To overcome the issues of current PL and photo-crosslinking techniques, we here introduce a new method that can perform a photo-crosslinking reaction with proximal proteins using a visible light-activable chemical ligand (Spotlight) in a live cell. For this reason, we utilized the HaloTag system to efficiently deliver AzNP to the POI. HaloTag is an engineered tag protein that can covalently capture the haloalkane ligand within a few minutes in live cells with high efficiency. Since protein-ligand binding interactions and various “in-cell chemical reactions,” including the strain-promoted click reaction and photo–activation reactions, have been successfully realized with HaloTag, we expected HaloTag to be a suitable platform for our proximity photo-crosslinking system using an AzNP-conjugated ligand.

Among the photo-crosslinkable handles, naphthyl azide-based 4-azido-N-ethyl-1,8-naphthalimide (AzNP) attracted our interest for the following reasons: (1) it is highly stable in aqueous solutions, and has been widely used in hydrogen sulfide sensors;17,18 (2) it emits strong green fluorescence, which has been used in the fluorogenic imaging of alkyne-modified biomolecules in live mammalian cells; and (3) it shows good photo-crosslinking ability: upon UV illumination, AzNP can convert to the aryl nitrene species, which can covalently attach to proteins. To test this model, we synthesized AzNP-conjugated HaloTag ligands (VL1 and VL2) with two linker sizes (see ESI†). VL1 showed fairly strong absorbance in the visible light range (λmax = 375 nm, extinction coefficient value = 2230 M−1 cm−1; Fig. S3†). In this model system, VL1 successfully generated the photo-crosslinked product of FKBP25-HaloTag and EGFP-FRB that appeared around 120 kDa only in the presence of rapamycin and in the blue LED light illumination condition. In this reaction on the FKBP25-HaloTag, VL1 containing the PEG1 linker showed stronger crosslinking efficiency with EGFP-FRB compared with that of VL2 containing the PEG2 linker. Notably, we used an ambient blue LED household lamp (∼0.057 W cm−2) for all of our photo-crosslinking experiments in test tubes and live cells with VL1, which highlights the sensitivity of AzNP and the requirement of only low-intensity visible light illumination. We tested the specificity of AzNP-containing HaloTag ligands (VL1) to the HaloTag protein and whether it captures the local PPI network in various subcellular compartments in live cells. Since VL1 emits green fluorescence (λmax = 540 nm, Fig. S3†) and its fluorescence is increased after the photo-crosslinking reaction (Fig. S4†), we expected that targeting of VL1 and formation of POI-HaloTag could be readily tracked in real time in live cells, whereas other UV-crosslinking ligands (e.g., phenyl azide, diazirine) would not be visualized with microscope imaging due to their negligible fluorescence emission.

> SGSAEIGTGFPFDPHYVEVLGERMHYVDVGPRDGTPVLFLHGNPTSSYVWRNIIPHVAPTHRCIAPDLIGMGKSDKPDLGYFFDDHVRFMDAFIEALGLEEVVLVIHDWGSALGFHWAKRNPERVKGIAFMEFIRPIPTWDEWPEFARETFQAFRTTDVGRKLIIDQNVFIEGTLPCGVVRPLTEVEMDHYREPFLNPVDREPLWRFPNELPIAGEPANIVALVEEYMDWLHQSPVPKLLFWGTPGVLIPPAEAARLAKSLPNCKAVDIGPGLNLLQEDNPDLIGSEIARWLSTLEISG>MSQAATPAADGKVKISIDPLTRVEGHLKIEVEVKDGKVVDAKCSGGMFRGFEQILRGRDPRDSSQIVQRICGVCPTAHCTASVMAQDDAFGVKVTTNGRITRNLIFGANYLQSHILHFYHLAALDYVKGPDVSPFVPRYANADLLTDRIKDGAKADATNTYGLNQYLKALEIRRICHEMVAMFGGRMPHVQGMVVGGATEIPTADKVAEYAARFKEVQKFVIEEYLPLIYTLGSVYTDLFETGIGWKNVIAFGVFPEDDDYKTFLLKPGVYIDGKDEEFDSKLVKEYVGHSFFDHSAPGGLHYSVGETNPNPDKPGAYSFVKAPRYKDKPCEVGPLARMWVQNPELSPVGQKLLKELYGIEAKNFRDLGDKAFSIMGRHVARAEETWLTAVAVEKWLKQVQPGAETYVKSEIPDAAEGTGFTEAPRGALLHYLKIKDKKIENYQIVSATLWNANPRDDMGQRGPIEEALIGVPVPDIKNPVNVGRLVRSYDPULGCAVH[2x];>[2x]MTEGAKKAPVIWVQGQGCTGCSVSLLNAVHPRIKEILLDVISLEFHPT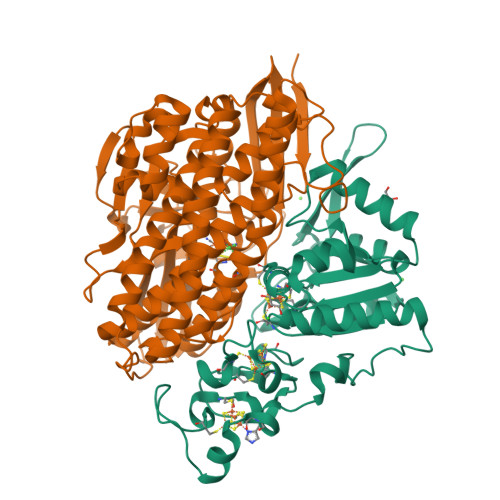VMASEGEMALAHMYEIAEKFNGNFFLLVEGAIPTAKEGRYCIVGETLDAKGHHHEVTMMELIRDLAPKSLATVAVGTCSAYGGIPAAEGNVTGSKSVRDFFADEKIEKLLVNVPGCPPHPDWMVGTLVAAWSHVLNPTEHPLPELDDDGRPLLFFGDNIHENCPYLDKYDNSEFAETFTKPGCKAELGCKGPSTYADCAKRRWNNGINWCVENAVCIGCVEPDFPDGKSPFYVAE>[2x]HTIFSSLEVNGVNQGLGEGVRVPTYNGPIEDVTSASIACNGSPNTVASTSKVITVQAGTNVTAIWRYMLSTTGDSPADVMDSSHKGPTIAYLKKVD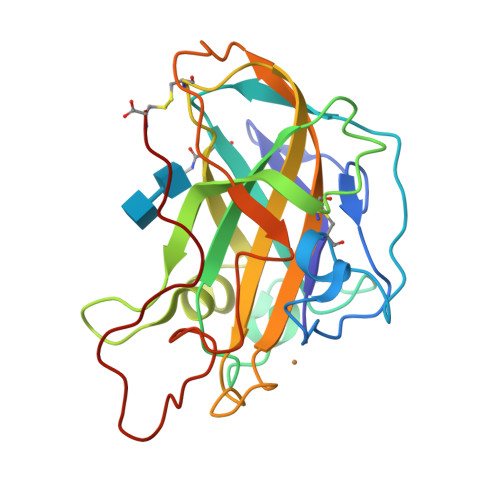NAATASGVGNGWFKIQQDGMDSSGVWGTERVINGKGRHSIKIPECIAPGQYLLRAEMIALHAASNYPGAQFYMECAQLNVVGGTGAKTPSTVSFPGAYSGSDPGVKISIYWPPVTSYTVPGPSVFTC>[6x]MIAHLINTDIGNRGVLKVYLDYRRKNFNFLHNSTKMFLDNLERVLIVTGFPIPPMMVAETDGPPGALAIYRAVEMLGGKAEILTYSEVEKALEPFGVSLARTPEPEDYSLIISVETPGRAADGRYYSMSALEIKRDPLDGIFLKARALGIPTIGVGDGGNEIGMGKIRELVVGH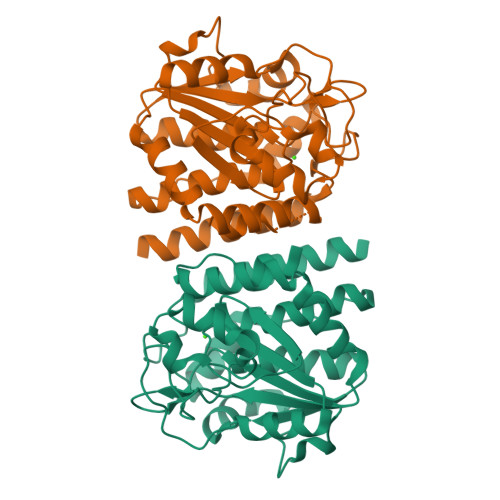VPHGEKIASVVETDELIVSAVSNWGAYGLVAQASIEVGRNLLEGWDERRVIEAISSAGLIDGVSKTLAPSVDGIRLMVHEGIVELLKAVVDEAIL> EAPYASLTEIEHLVQSVCKSYRETCQLRLEDLLRQRSNIFSREEVTGYQRKSMWEMWERCAHHLTEAIQYVVEFAKRLSGFMELCQNDQIVLLKAGAMEVVLVRMCRAYNADNRTVFFEGKYGGMELFRALGCSELISSIFDFSHSLSALHFSEDEIALYTALVLINAHRPGLQEKRKVEQLQYNLELAFHHHLCKTHRQSI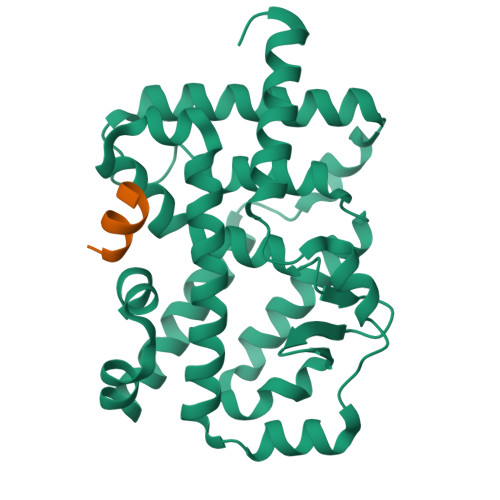LAKLPPKGKLRSLCSQHVERLQIFQHLHPIVVQAAFPPLYKELFSTETESPVGLSK;> RHKILHRLLQEGSPS> SMFPRGRPQDSVNVDAVISKIESTFARFPHERATMDDMGLVAKACGCPLYWKGPLFYGAGGERTGSVSVHKFVAMWRKILQNCHDDAAKFVHLLMSPGCNYLVQEDFVPFLQDVVNTHPGLSFLKEASEFHSRYITTVIQRIFYAVNRSWSGRITCAELRRSSFLQNVALLEEEADINQLTEFFSYEHFYVIYCKFWELDTDHDLLIDADDLARHNDHALSTKMIDRIFSGA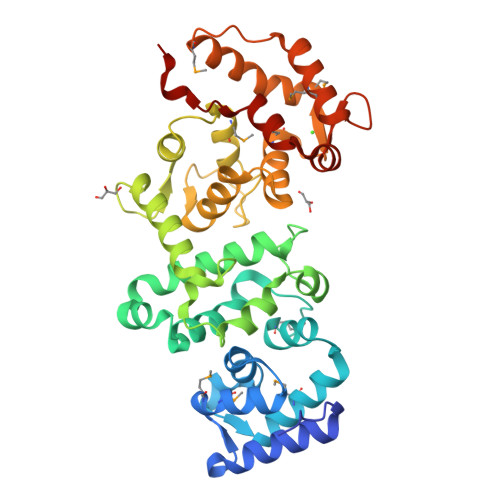VTRGRKVQKEGKISYADFVWFLISEEDKKTPTSIEYWFRCMDLDGDGALSMFELEYFYEEQCRRLDSMAIEALPFQDCLCQMLDLVKPRTEGKITLQDLKRCKLANVFFDTFFNIEKYLDHEQK> MPLAFCGTENHSAAYRVDQGVLNNGCFVDALNVVPHVFLLFITFPILFIGWGSQSSKVHIHHSTWLHFPGHNLRWILTFILLFVLVCEIAEGILSDGVTESRHLHLYMPAGMAFMAAITSVVYYHNIETSNFPKLLIALLIYWTLAFITKTIKFVKFYDHAIGFSQLRFCLTGLLVILYGMLLLVEVNVIRVRRYIFFKTPREVKPPEDLQDLGVRFLQPFVNLLSKGTYWWMNAFIKTAHKKPIDLRAIAKLPIAMRALTNYQRLCVAFDAQARKDTQSPQGARAIWRALCHAFGRRLILSSTFRILADLLGFAGPLCIFGIVDHLGKENHVFQPKTQFLGVYFVSSQEFLGNAYVLAVLLFLALLLQRTFLQASYYVAIETGINLRGAIQTKIYNKIMHMSTSNLSMGEMTAGQICNLVAIDTNQLMWFFFLCPNLWTMPVQIIVGVILLYYILGVSALIGAAVIILLAPVQYFVATKLSQAQRTTLEHSNERLKQTNEMLRGMKLLKLYAWESIFCSRVEVTRRKEMTSLRAFAVYTSISIFMNTAIPIAAVLITFVGHVSFFKESDLSPSVAFASLSLFHILVTPLFLLSSVVRSTVKALVSVQKLSEFLSSAEIREEQCAPREPAPQGQAGKYQAVPLKVVNRKRPAREEVRDLLGPLQRLAPSMDGDADNFCVQIIGGFFTWTPDGIPTLSNITIRIPRGQLTMIVGQVGCGKSSLLLATLGEMQKVSGAVFWNSNLPDSEGEDPSSPERETAAGSDIRSRGPVAYASQKPWLLNATVEENITFESPFNKQRYKMVIEACSLQPDIDILPHGDQTQIGERGINLSGGQRQRISVARALYQQTNVVFLDDPFSALDVHLSDHLMQAGILELLRDDKRTVVLVTHKLQYLPHADWIIAMKDGTIQREGTLKDFQRSECQLFEHWKTLMNRQDQELEKETVMERKASEPSQGLPRAMSSRDGLLLDEEEEEEEAAESEEDDNLSSVLHQRAKIPWRACTKYLSSAGIL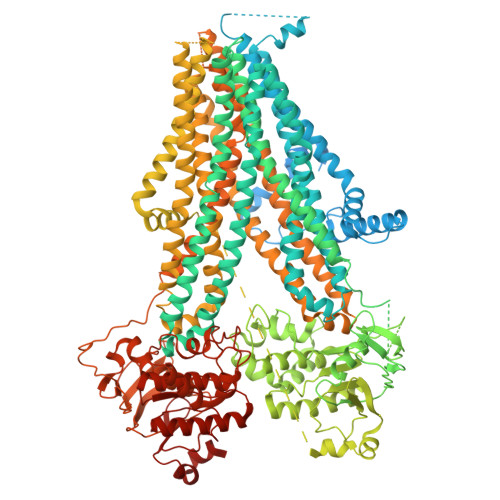LLSLLVFSQLLKHMVLVAIDYWLAKWTDSALVLSPAARNCSLSQECDLDQSVYAMVFTLLCSLGIVLCLVTSVTVEWTGLKVAKRLHRSLLNRIILAPMRFFETTPLGSILNRFSSDCNTIDQHIPSTLECLSRSTLLCVSALTVISYVTPVFLVALLPLAVVCYFIQKYFRVASRDLQQLDDTTQLPLVSHFAETVEGLTTIRAFRYEARFQQKLLEYTDSNNIASLFLTAANRWLEVCMEYIGACVVLIAAATSISNSLHRELSAGLVGLGLTYALMVSNYLNWMVRNLADMEIQLGAVKRIHALLKTEAESYEGLLAPSLIPKNWPDQGKIQIQNLSVRYDSSLKPVLKHVNTLISPGQKIGICGRTGSGKSSFSLAFFRMVDMFEGRIIIDGIDIAKLPLHTLRSRLSIILQDPVLFSGTIRFNLDPEKKCSDSTLWEALEIAQLKLVVKALPGGLDAIITEGGENFSQGQRQLFCLARAFVRKTSIFIMDEATASIDMATENILQKVVMTAFADRTVVTIAHRVHTILSADLVMVLKRGAILEFDKPETLLSQKDSVFASFVRADK> MVEATAQETDRPRFSFSIAAREGKARTGTIEMKRGVIRTPAFMPVGTAATVKALKPETVRATGADIILGNTYHLMLRPGAERIAKLGGLHSFMGWDRPILTDSGGYQVMSLSSLTKQSEEGVTFKSHLDGSRHMLSPERSIEIQHLLGSDIV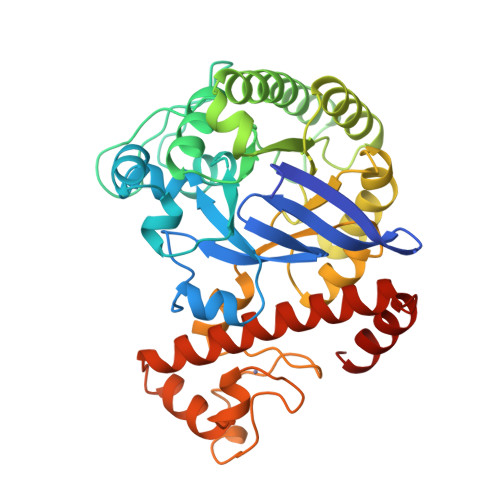MAFYECTPYPATPSRAASSMERSMRWAKRSRDAFDSRKEQAENAALFGIQQGSVFENLRQQSADALAEIGFDGYAVGGLAVGEGQDEMFRVLDFSVPMLPDDKPHYLMGVGKPDDIVGAVERGIDMFDCVLPTRSGRNGQAFTWDGPINIRNARFSEDLKPLDSECHCAVCQKWSRAYIHHLIRAGEILGAMLMTEHNIAFYQQLMQKIRDSISEGRFSQFAQDFRARYFARNS>[4x]MSTAEPAPDPTNPSTSGLAPTTNGIGSPPPTASAATKFSILTKFLRRKNQVHTTTAQQNEFMQKYMPNGNSNAVQPAATGGQPASSDGGSAIEVPPPKESYAVRIRKYLANYTQDPSTDNFYYWTCVVTVAYIYNLLFVIARQVFNDLIGPSSQSLCRFYNGTLNSTTQVECTYNMLTNMKEMPTYSQYPDLGWSKYWHFRMLWVFFDLLMDCVYLIDTFLNYRMGYMDQGLVVREAEKVTKAYWQSKQYRIDGISLIPLDYILGWPIPYINWRGLPILRLNRLIRYKRVRNCLERTETRSSMPNAFRVVVVVWYIVIIIHWNACLYFWISEWIGLGTDAWVYGHLNKQSLPDDITDTLLRRYVYSFYWSTLI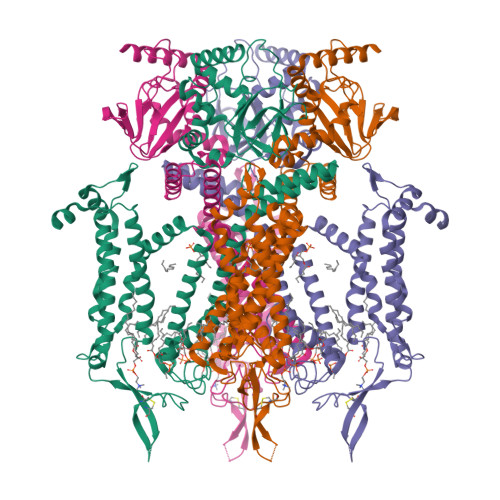LTTIGEVPSPVRNIEYAFVTLDLMCGVLIFATIVGNVGSMISNMSAARTEFQNKMDGIKQYMELRKVSKQLEIRVIKWFDYLWTNKQSLSDQQVLKVLPDKLQAEIAMQVHFETLRKVRIFQDCEAGLLAELVLKLQLQVFSPGDFICKKGDIGREMYIVKRGRLQVVDDDGKKVFVTLQEGSVFGELSILNIAGSKNGNRRTANVRSVGYTDLFVLSKTDLWNALREYPDARKLLLAKGREILKKDNLLDENAPEEQKTVEEIAEHLNNAVKVLQTRMARLIVEHSSTEGKLMKRIEMLEKHLSRYKALARRQKTMHGVSIDGGDISTDGVDERVRPPRLRQTKTIDLPTGTESESLLK(2~{S})-2-(aminocarbonylamino)-3-(4-hydroxyphenyl)propanoic 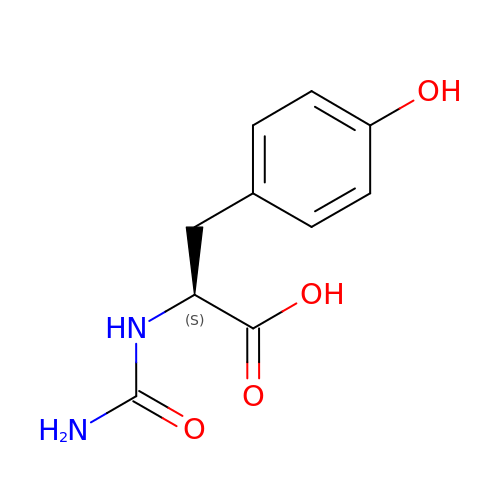acid | C10 H12 N2 O4 | PNLKYZVGQWCHBH-QMMMGPOBSA-N> AHLESLTHPGSKVTFPIDQDISATPQNPNLKVFFFDIDNCLYKSSTRIHDLMQQSILRFFQTHLKLSPEDAHVLNNSYYKEY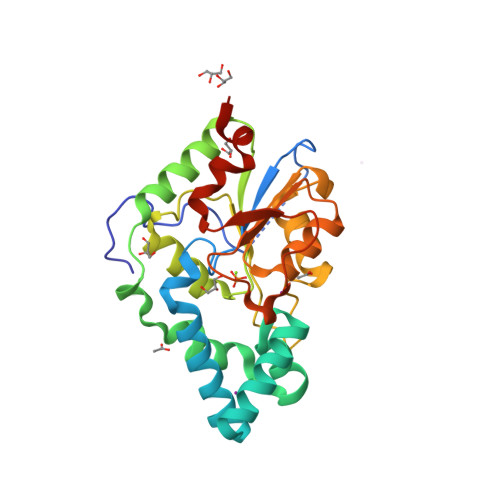GLAIRGLVMFHKVNALEYNRLVDDSLPLQDILKPDIPLRNMLLRLRQSGKIDKLWLFTNAYKNHAIRCLRLLGIADLFDGLTYCDYSRTDTLVCKPHVKAFEKAMKESGLARYENAYFIDDSGKNIETGIKLGMKTCIHLVENEVNEILGQTPEGAIVISDILELPHVVSDLFLEHHHHHH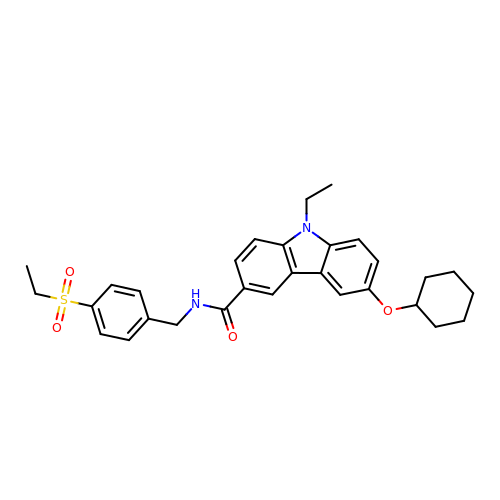6-cyclohexyloxy-9-ethyl-~{N}-[(4-ethylsulfonylphenyl)methyl]carbazole-3-carboxamide | C30 H34 N2 O4 S | XJCREIMPADNIDU-UHFFFAOYSA-N>MGSYLHEPPGDEPSMRIEQPKTADRAPEQVAIHICEPSKVVTESFPFSETAEPEAKSKNCPCPEIARIGPCPNKPPKIPINRGLSRISTNKSRPKSRFGEPSWPVESSLDLTSQSPVSPYREEAFSVENCGTAGSRRGSFARGTTSRAASSSRKDETKEGPDEKEVYQRVTAQLSARNQKRMTVKLMIELSVFLCLLGCLVCSLTVDGFKRYTVIGLDIWKWFLLLLVIFSGMLITHWIVHVAVFFVEWKFLMRKNVLYFTHGLKTSVEVFIWITVVLATWVMLIKPDVNQPHQTRKILEFVTWTIVTVLIGAFLWLVKTTLLKILASSFHLNRFFDRIQESVFHHSVLQTLAGRPVVELAQGISRTESQDGAGQVSFMEHTKTQNKKVVDVGKLHQMKQEKVPAWTMQLLVDVVSNSGLSTMSGMLDEDMVEGGVELDDDEITNEEQAIATAVRIFDNIVQDKVDQSYIDRVDLHRFLIWEEVDHLFPLFEVNEKGQISLKAFAKWVVKVYNDQAALKHALNDNKTAVKQLNKLVTAILIVMMIVIWLIVTGIATTKLIVLLSSQLVVAAFIFGNTCKTIFEAIIFVFVMHPFDVGDRCVIDGNKMLVEEMNILTTVFLKWDKEKVYYPNSILCTKAIGNFFRSPDQGDVLEFSVDFTTPVLKIGDLKDRIKMYLEQNLNFWHPQHNMVVKEIENVNKIKMALFVNHTINFQDFAEKNR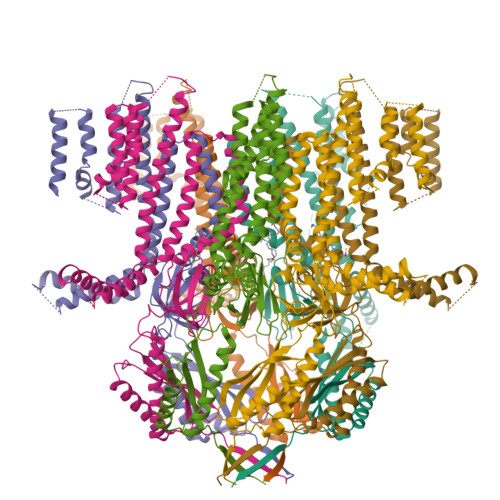RRSELVLELKKIFEELDIKYNLLPQEISIRNMGSGSLEVLFQ[7x]> MSNEDYGYDYDYLFKIVLIGDSGVGKSNLLSRFTTDEFNIESK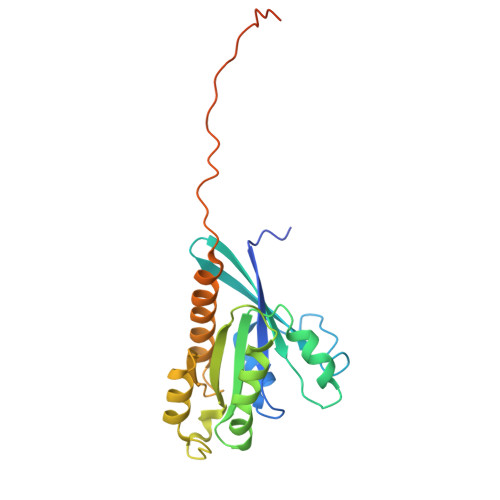STIGVEFATRTIEVENKKIKAQIWDTAGQERYRAITSAYYRGAVGALIVYDISKSSSYENCNHWLTELRENADDNVAVGLIGNKSDLAHLRAVPTDEAKNFAMENQMLFTETSALNSDNVDKAFRELIVAIFQMVSKHQVDLSGSGTNNMGSNGAPKGPTISLTPAPKEDKKKKSSNCC>PQKICLICGDEASGCHYGVLTCGS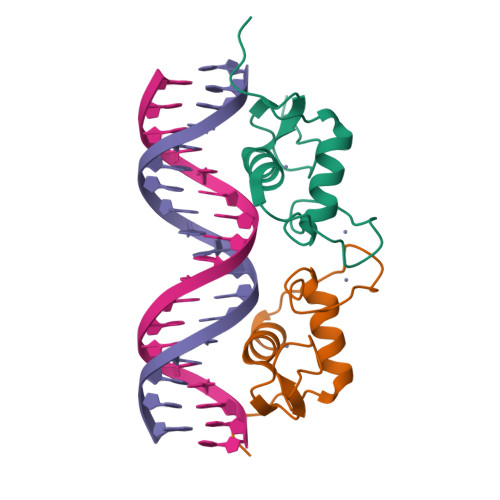CKVFFKRAMEGQHNYLCAGRNDCIVDKIRRKNCPACRLRKCCQAGMVLGGRKFK[2x]>[4x]MAE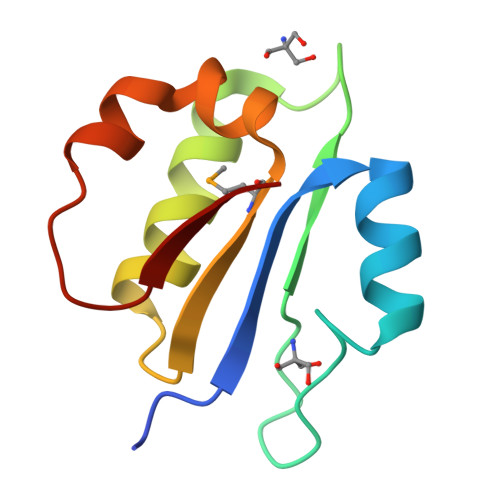KRTLIAVIADEDTTTGLLLAGIGQITPETQEKNFFVYQEGKTTKEEITDKFNHFTEERDDIAILLMNQHIAENIRARVDSFTNAFPAILEI> GIDELWKGSYLDPTIGAKQKEANAVAGDAWPACLLRMKSFEDLHKLWYICLKEKNLLMGERWAARQHKQEMKQPERLQKVRRTMRRIL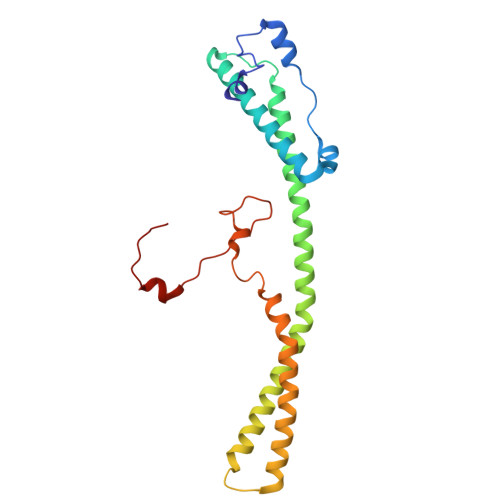IVLTKREIQQQCLRAKDILAKQQKREALETRRFQLEEKMLQLEHRIRRMEPAQSLQKEAWQATLDRYRSDHEDILIQLHPLRKETTQLLAPDWRYERKYSDLPGPIRWKKQYIPALEDQYRKPIRF> QQVCTQQAETHPPLTWQKCTASGCTPQQGSVVLDANWRWTHDTKSTTNCYDGNTWSSTLCPDDATCAKNCCLDGANYSGTYGVTTSGDALTLQFVTASNVGSRLYLMANDSTYQEFTLSGNEFSFDVDVSQLPCGLNGALYFVSMDADGGQSKYPGNAAGAKYGTGYCDSQCPRDLKFINGQANVEGWEPSSNNANTGVGGHGSCCSEMDIWEANSISEALTPHPCETVGQTMCSGDSCGGTYSNDRYGGTCD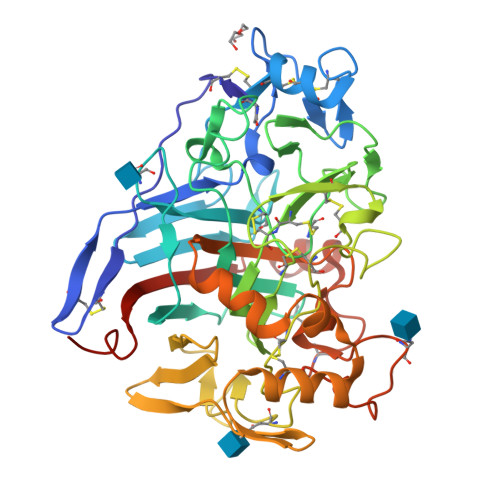PDGCDWNPYRLGNTSFYGPGSSFALDTTKKLTVVTQFATDGSISRYYVQNGVKFQQPNAQVGSYSGNTINTDYCAAEQTAFGGTSFTDKGGLAQINKAFQGGMVLVMSLWDDYAVNMLWLDSTYPTNATASTPGAKRGSCSTSSGVPAQVEAQSPNSKVIYSNIRFGPIGSTGGNTGSN3-(2-aminoquinolin-3-yl)-N-cyclohexyl-N-methylpropanamide | C19 H25 N3 O 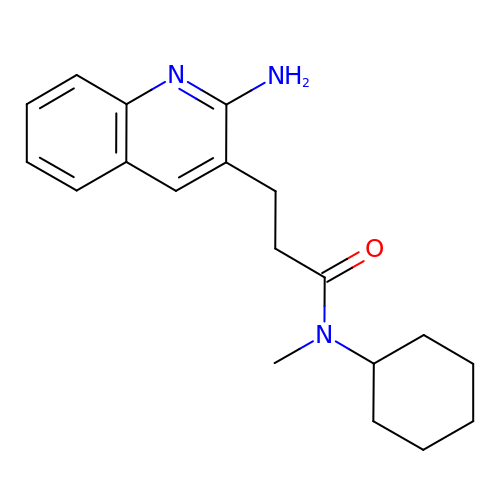| GRFOHUBBUMAJMM-UHFFFAOYSA-N>STVVTTESGLKYEDLTEGSGAEARAGQTVSVHYTGWLTDGQKFDSSKDRNDPFAFVLGGGMVIKGWDEGVQGMKVGGVRRLTIPPQLGYGAGGAGGVIPPNATLVFE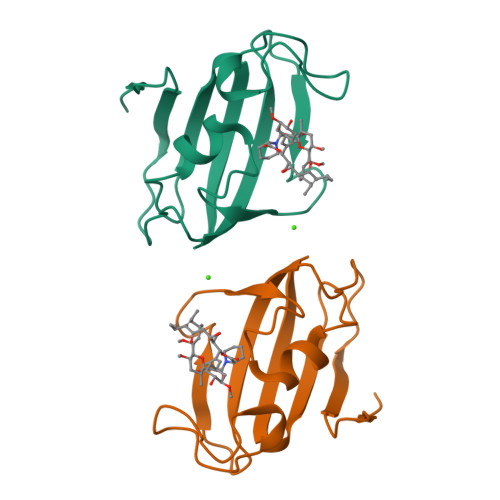VELLDV[2x]> MVKRTVATNGDASGAHRAKKMSKTHASHIINAQEDYKHMYLSVQPLDIFCWGTGSMCELGLGPLAKNKEVKRPRLNPFLPRDEAKIISFAVGGMHTLALDEESNVWSWGCNDVGALGRDTSNAKEQLKDMDADDSSDDEDGDLNELESTPAKIPRESFPPLAEGHKVVQLAATDNMSCALFSNGEVYAWGTFRCNEGILGFYQDKIKIQKTPWKVPTFSKYNIVQLAPGKDHILFLDEEGMVFAWGNGQQNQLGRKVMERFRLKTLDPRPFGLRHVKYIASGENHCFALTKDNKLVSWGLNQFGQCGVSEDVEDGALVTKPKRLALPDNVVIRSIAAGEHHSLILSQDGDLYSCGRLDMFEVGIPKDNLPEYTYKDVHGKARAVPLPTKLNNVPKFKSVAAGSHHSVAVAQNGIAYSWGFGETYAVGLGPFEDDTEVPTRIKNTATQDHNIILVGCGGQFSVSGGVKLSDEDAEKRADEMDD;> MDNGTDSSTSKFVPEYRRTNFKNKGRFSADELRRRRDTQQVELRKAKRDEALAKRRNFIPPTDGADSDEEDESSVSADQQFYSQLQQELPQMTQQLNSDDMQEQLSATVKFRQILSREHRPPIDVVIQAGVVPRLVEFMRENQPEMLQLEAAWALTNIASGTSAQTKVVVDADAVPLFIQLLYTGSVEVKEQAIWALGNVAGDSTDYRDYVLQCNAMEPILGLFNSNKPSLIRTATWTLSNLCRGKKPQPDWSVVSQALPTLAKLIYSMDTETLVDACWAISYLSDGPQEAIQAVIDVRIPKRLVELLSHESTLVQTPALRAVGNIVTGNDLQTQVVINAGVLPALRLLLSSPKENIKKEACWTISNITAGNTEQIQAVIDANLIPPLVKLLEVAEYKTKKEACWAISNASSGGLQRPDIIRYLVSQGCIKPLCDLLEIADNRIIEVTLDALENILKMGEADKEARGLNINENADFIEKAGGMEKIFNCQQNENDKIYEKAYKIIETYFGEEEDAVDETMAPQNAGNTFGFGSNVNQQFNFN

Eukaryotic cells maintain an intracellular gradient of the small GTPase Ran that is predominantly bound to GTP in the nucleus and GDP in the cytoplasm. This gradient is generated by the asymmetric distribution of Ran effectors: the guanine exchange factor RCC1 (regulator of chromatin condensation 1) is sequestered in the nucleus bound to chromatin, while the GTPase-activating protein specific for Ran, RanGAP, and various accessory Ran-binding proteins (RanBPs) reside in the cytoplasm. The association between importin α and β is mediated by the N-terminal importin β-binding (IBB) domain10 of importin α, which also binds NLS cargos via a C-terminal helical core composed of 10 Armadillo repeats (the ‘Arm-core’). Two NLS-binding pockets known as ‘major’ and ‘minor’ have been identified on the concave surface of importin α, spanning Arm repeats 2–4 and 6–8, respectively.

Unlike humans that express seven isoforms of importin α, Saccharomyces cerevisiae has only one importin α gene encoding Kap60. To determine how Kap60 binds the yeast homolog of mammalian RCC1 (Prp20p, herein referred to as yRCC1), we co-expressed the two proteins in bacteria, purified a homogeneous 1:1 complex and obtained large orthorhombic crystals of the Kap60:yRCC1 complex, which diffracted X-rays to high resolution. Difference maps revealed strong electron density at the N terminus of the β-propeller, which allowed us to model yRCC1 residues at the major and minor NLS-binding sites of Kap60 (residues 41–47 and 3–6, respectively). Unexpectedly, in the yeast complex the β-propeller is positioned onto the surface of Arms 1–2 of Kap60, making the complex more elongated and slender than the human counterpart (~135 vs. ~115 Å). First, at the minor NLS-binding pocket, yRCC1 residues K3 and R4 make close contacts at positions P1′ and P2′ of Kap60. The NLS major box of yRCC1 is unusual (17-RAKKMSK-23), lacking basic residues at both P3 and P4, but with R17 at position P−1 that makes a strong bidentate contact with D276. Third, a ‘loop-helix’ motif (residues 24–46) lies immediately C-terminal of the yRCC1 major NLS box and connects it to the first β-strand of the β-propeller (residues 47–51). While the loop (residues 24–32) makes no contacts with Kap60, the short α-helix (residues 33–40) packs against helixes B of Arms 1–2, sandwiched between the yRCC1 β-propeller and the concave groove of Kap60. The α-helix in yRCC1 is not present in human RCC1, where the linker is 13 residues shorter than in yeast. Mutations in this motif did not destabilize yRCC1 binding to Kap60, suggesting it functions like a “spacer” rather than a binding determinant, used to position the β-propeller onto the N terminus of Kap60 and avoid steric clashes with the Arm-core.>GAMTGVISSSSIGEKINEWYMYIRRFSIPDAEYLRREIKQELDQMEEDQDLHLYYSLMEFRHNLMLEYLEPLEKMRIEEQPRLSDLLLEIDKKQARLTGLLEYYFNFFRGMYELDQREYLSAIKFFKKAESKLIFVKDRIEKAEFFFKMSESYYYMKQTYFSMDYARQAYEIYKEHEAYNIRLLQCHSLFATNFLDLKQYEDAISHFQKAYSMAEAEKQPQLMGRTLYNIGLCKNSQSQYEDAIPYFKRAIAVFEESNILPSLPQAYFLITQIHYKLGKIDKAHEYHSKGMAYSQKAGDVIYLSEFEFLKSLYLSGPDEEAIQGFFDFLESKMLYADLEDFAIDVAKYYHERKNFQKASAYFLKVEQVRQLIQGGVSLYEIEV[2x]

In Bacillus, the Rap protein family modulates complex signaling processes mediated by two-component systems, such as competence, sporulation, or biofilm formation, by inhibiting the RR components involved in these pathways. The second subgroup, comprising RapC, RapF, RapG, RapH, and RapK, blocks the action of the target RR by a direct interaction with their DNA binding domain, and works as an anti-activator. For Rap proteins, regulatory peptides are called Phr and their mature active form is a penta- or hexa-peptide generated from a ∼40 amino-acid precursor by means of a post-transcriptional export-import process. As previously disclosed by the crystal RapF structure in complex with the DNA-binding domain of its RR target ComA, RapF was an all-helical protein consisting of two domains: a small N-terminal 3-helix bundle domain (residues 1–68) and a large C-terminal TPR domain (residues 98–370), both connected by a linker region (69–97).

In order to determine the molecular basis of RapF inhibition by Phr peptides, the X-ray structures of RapF alone and in complex with its inhibitory pentapeptide PhrF (QRGMI) were determined. The crystal asymmetric unit showed two molecules in the free RapF structure and one RapF molecule bound to one PhrF peptide in the structure of the complex. The structural models for the free and PhrF complex forms were refined to a final resolution of 2.25 and 3.1 Å, respectively. A comparison of the free RapF and the RapF-ComA structure reveals that binding of ComA to RapF only promoted slight local conformational changes in RapF, which were mainly restricted to the RR recognition domain (the 3-helix bundle plus the linker region; 1–97) in order to bind the DNA binding helix of ComA. The core TPR domains remained at the same position (root mean square = 0.66 Å for the superimposition of residues 98–380), which supports that RapF in solution presents an active conformation that is competent to bind ComA. When RapF was free or in complex with ComA, the 3-helix bundle domain was projected apart from the TPR domain, thus exposing the ComA binding surface. The RapF TPR domain folded in a large superhelix to generate a pseudo circular structure that was closed in a wide channel (8,588 Å3, calculated by the CASTp software) by the interaction of the terminal part of TPR7 (and the following C-terminal tail) with the initial part of TPR1. As a channel, the generated ring-like structure was open on both faces. Arg80 was located in a loop of the linker region, participated in the ComA binding and was exposed to the solvent in the RapF free from.>[2x]MIKKILIANRGEIAVRIVRACSEMGIKSVAIYSDADRHALHVKKADEAYNIGSDPVLGYLNAHNIVNLAVASGCDALHPGYGFLSENPELAEICARRGIKFIGPDAKVIRQMGDKIQARTAMIKAGIPCVGSSGVVNPRHIEVQVLADSHGNVIHLFERDCSIQRRN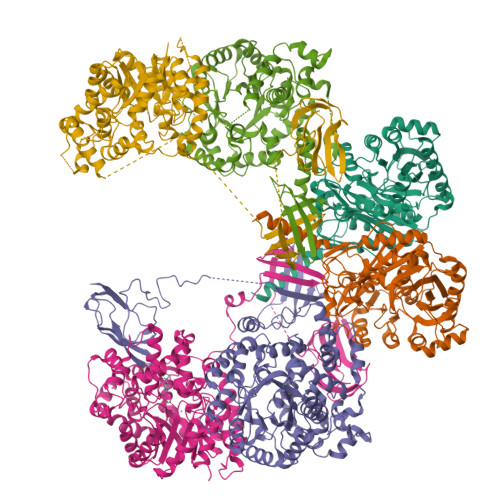QKLIEIAPSPQLSKAQREYIGNLAVKAAKAVGYKNAGTVEFLLDSDNNFYFMEMNTRLQVEHTVTEQITGIDIVQEQIRVADGQRLQYKQSEVQYRGFAMEFRINAEDPKNDFLPSFGKITRYYAPGGPGIRMDAAMYSGYVIPPYYDSMCAKLTVWALNWESVVERGRRALNDTVVYGVKTTIPYYQEILKHPDFRNAIFNTSFVESHPELANYATQFPRELVAAAISAAIAAHEGI;>[4x]MAKVHVTDVVLRDGHQSLIATRMRTDDMLPICSKLDAVGYWSLEAWGGATFDACVRYLREDPWERLKKLRKALPNSRLQMLLRGQNLLGYRHYSDDVVRAFVQKSADNGIDVFRIFDAMNDLRNLKVSIESVKAVGKHAEGTISYTTSPVHDIPYFVNLAKELESFGCDTIAIKDMASLLTPQVTGDLVKALREAVSLPIHLHAHATSGLASMSIQRAVDNGVAIVDGCISSFAEGASLPATESIVAALKGTEYDTGLDIGLLQEISAYFREVRKKYWQFESEFTGVDTRVLVNQVPGGMISNLSNQLKEQGALDRMDAVLDEIPRVREDLGYPPLVTPTSQIVGTQAVLNVMTGARYKSVTNEVKNYLLGHYGKAPSTVNPDVRNLAVGNAQVIECRPADLLTAEMEKLRNEVEGLAASAADVLTYAMFPDLAKTFLQERNAGSLKPEPLLDKEAVTSRESHSRFAPTEFNVTLHGETFHIKLTGSGHHGEEQRPFYVSVDGVTEEVVVEILNEIEVSGGGQSSGEAKRKASSAASSGRPRPTHAGCVTTAMPGTIVDVKVNVGDKVSAGDAVLVIEAMKMENEIQASKSGVVVAINVKKGDSVTPDEALLEIQPD> MENTENSVDSKSIKNLEPKIIHGSESMDSGISLDNSYKMDYPEMGLCIIINNKNFHKSTGMTSRSGTDVDAANLRETFRNLKYEVRNKNDLTREEIVELMRDVSKEDHSKRSSFVC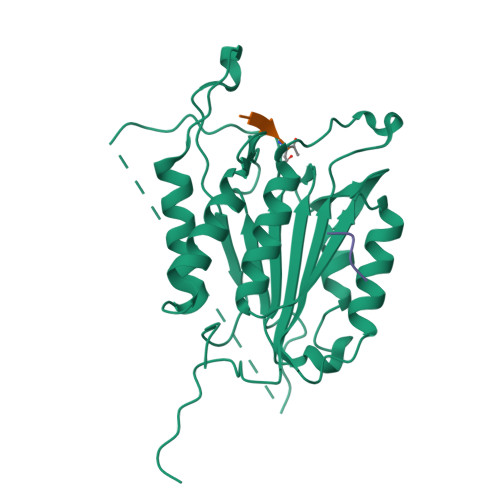VLLSHGEEGIIFGTNGPVDLKKITNFFRGDRCRSLTGKPKLFIIQACRGTELDCGIETDSGVDDDMACHKIPVEADFLYAYSTAPGYYSWRNSKDGSWFIQSLCAMLKQYADKLEFMHILTRVNRKVATEFESFSFDATFHAKKQIPCIQSMLTKELYFYH;> DDDM> MES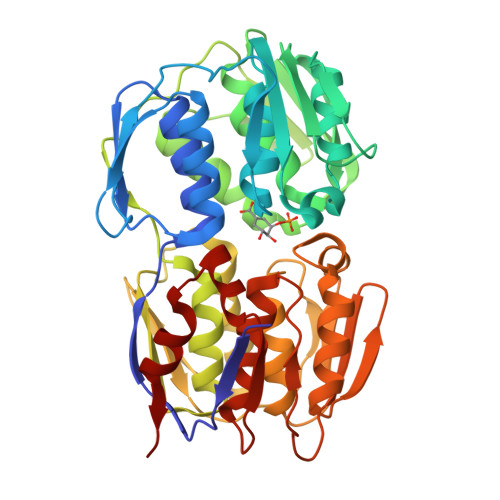LTLQPIARVDGTINLPGSKSVSNRALLLAALAHGKTVLTNLLDSDDVRHMLNALTALGVSYTLSADRTRCEIIGNGGPLHAEGALELFLGNAGTAMRSLAAALCLGSNDIVLTGEPRMKERPIGHLVDALRLGGAKITYLEQENYPPLRLQGGFTGGNVDVDGSVSSQFLTALLMTAPLAPEDTVIRIKGDLVSKPYIDITLNLMKTFGVEIENQHYQQFVVKGGQSYQSPGTYLVEGDASSASYFLAAAAIKGGTVKVTGIGRNSMQGDIRFADVLEKMGATICWGDDYISCTRGELNAIDMDMNHIPDAAMTIATAALFAKGTTTLRNIYNWRVKETDRLFAMATELRKVGAEVEEGHDYIRITPPEKLNFAEIATYNDHRMAMCFSLVALSDTPVTILDPKCTAKTFPDYFEQLARISQAA>[2x]GKLSLQDVAELIRARACQRVVVMVGAGISTPSGIPDFRS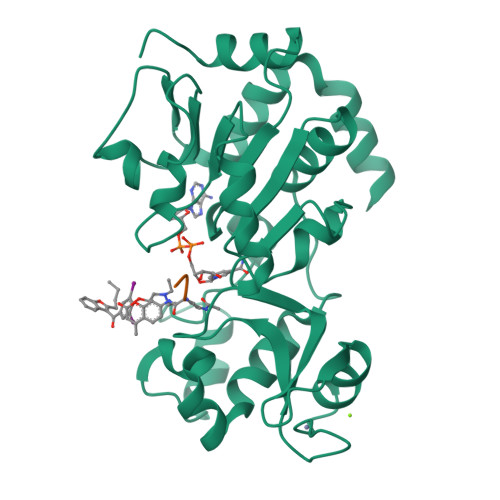PGSGLYSNLQQYDLPYPEAIFELPFFFHNPKPFFTLAKELYPGNYKPNVTHYFLRLLHDKGLLLRLYTQNIDGLERVSGIPASKLVEAHGTFASATCTVCQRPFPGEDIRADVMADRVPRCPVCTGVVKPDIVFFGEPLPQRFLLHVVDFPMADLLLILGTSLEVEPFASLTEAVRSSVPRLLINRDLVGPLAWHPRSRDVAQLGDVVHGVESLVELLGWTEEMRDLVQRET;>RHKK[2x]>NYLFEYAPDVLESFPNKHVNRDYFVKFNCPEFTSLCPKTGQPDFATIYISYIPDEKMVESKSLKLYLFSFRNHGDFHQDCMNIIMNDLIELMDPRYIEVWGKFTPRGGISIDPYTNYGKPGTKYEKMAEYRMMNHDLYPETIDNR[5x]

QueF is the nicotinamide adenine dinucleotide phosphate (NADPH)-dependent nitrile reductase that functions in the biosynthetic pathway of the tRNA-modified nucleoside queuosine (Q,), a 7-deazaguanosine nucleoside found at the wobble position of bacterial and eukaryotic tRNAs possessing the GUN anticodon (those encoding for Tyr, His, Asp and Asn). QueF catalyzes the NADPH-dependent 4-electron reduction of the nitrile group of the pathway intermediate 7-cyano-7-deazaguanine (preQ0) to 7-aminomethyl-7-deazaguanine (preQ1), the last intermediate in the tRNA-independent portion of the pathway. QueF belongs to the tunnelling fold (T-fold) structural superfamily of purine/pterin binding proteins. B. subtilis QueF, a ~160 amino acid protein with a single T-fold domain, is a homodecamer of two head-to-head facing pentamers, each composed of a cyclic arrangement of monomeric T-fold subunits, forming a tunnel in the center.

The Glu97Gln mutant enzyme crystallized in the same space group (P3221) as previously determined for the wild-type enzyme and the Cys55Ala mutant, both bound to preQ0. The refined structure contains five subunits (A–E) in the crystallographic asymmetric unit and exhibits good geometry and an R factor below 0.2. The overall structure shows a homodecamer formed by two pentameric subunits organized in a face-to-face manner through coordination of the C-terminal tails via divalent metal ions, similar to the preQ0-bound structures. However, the Glu97Gln mutant structure is substantially more symmetric, and represents the substrate- and cofactor-free form of the enzyme (here referred to as the apo form) as no difference electron density corresponding to the substrate, cofactor or the product is seen in any of the ten active sites in the homodecamer. Superposition of the Glu97Gln mutant structure with any of the preQ0-bound structures (wild-type or Cys55Ala) reveals significant tightening of the homodecamer in the apo form relative to the preQ0-bound form. The most striking difference is the formation of a disulfide bridge in all the active sites between the catalytic Cys55 and Cys99 located in the N-terminal turn of the second helix of the tunnel fold, the helix lining the inter-subunit interface. Disulfide formation is accompanied by full unwinding of the N-terminal turn of the helix, indicating conformational flexibility of the active sites. All of the disulfides in the protein decamer exhibit dihedral angles with the signs −,−,−,+,− for χ1, χ2, χ3, χ2′, χ1′, respectively, indicating a minus left-handed hook (–LHHook) geometry characteristic of regulatory disulfides. These angles and the calculated disulfide strain energy of ~13–19 kJ/mol suggest an allosteric regulatory function, rather than a catalytic or structural function, for the active site disulfides of QueF.> MGITKEEVNSYYQKAGIVLTDEEVDQIQLMDYGLGKERKVGLQLF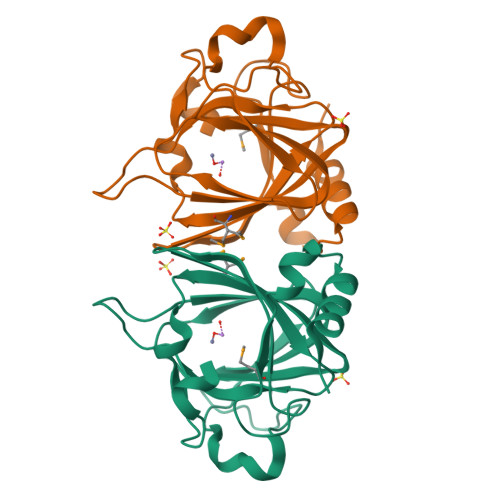VYVNTDRYCSKELVLFPGQTCPEHRHPPVDGQEGKQETFRCRYGKVYLYVEGEKTPLPKVLPPQEDREHYTVWHEIELEPGGQYTIPPNTKHWFQAGEEGAVVTEMSSTSTDKHDIFTDPRILEHHHHHH>[10x]APADNAADARPVDVSVSIFINKIYGVNTLEQTYKVDGYIVAQWTGKPRKTPGDKPLIVENTQIERWINNGLWVPALEFINVVGSPDTGNKRLMLFPDGRVIYNARFLGSFSNDMDFRLFPFDRQQFVLELEPFSYNNQQLRFSDIQVYTENIDNEEIDEWWIRGKASTHIS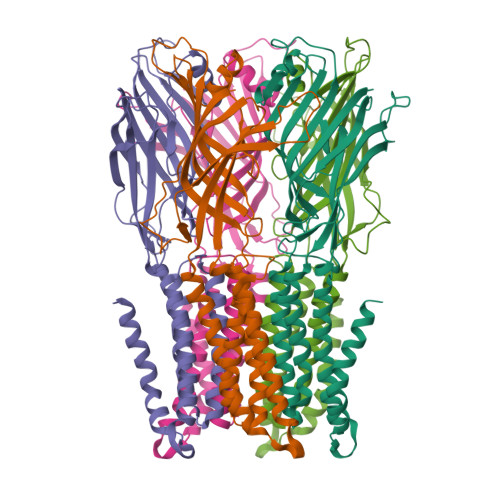DIRYDHLSSVQPNQNEFSRITVRIDAVRNPSYYLWSFILPLGLIIAASWSVFWLESFSERLQTSFTLMLTVVAYAFYTSNILPRLPATTVIDQMIIAGYGSIFAAILLIIFAHHRQANGVEDDLLIQRCRLAFPLGFLAIGCVLVIRGITL>MTDQATPNLPSRDFDSTAAFYERLGFGIVFRDAGWMILQRGDLMLEFFAHPGLDP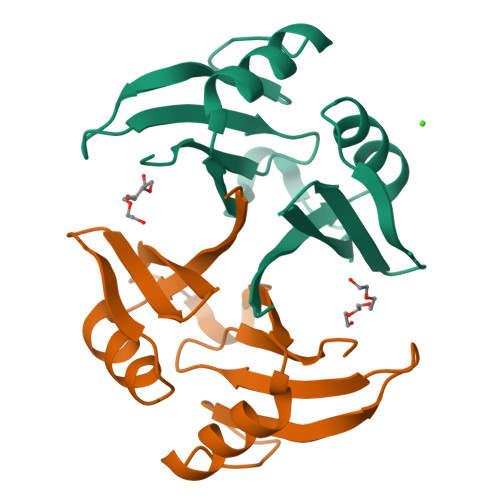LASWFSCCLRLDDLAEFYRQCKSVGIQETSSGYPRIHAPELQGWGGTMAALVDPDGTLLRLIQNELLAGIS[2x]>[8x]GNSITSATDEQPHIGNYRLQKTIGKG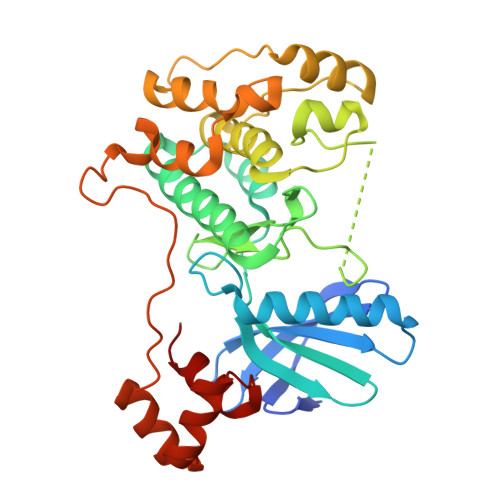NFAKVKLARHVLTGREVAVKIIDKTQLNPTSLQKLFREVRIMKILNHPNIVKLFEVIETEKTLYLVMEYASGGEVFDYLVAHGRMKEKEARAKFRQIVSAVQYCHQKYIVHRDLKAENLLLDGDMNIKIADFGFSNEFTVGNKLDTFCGSPPYAAPELFQGKKYDGPEVDVWSLGVILYTLVSGSLPFDGQNLKELRERVLRGKYRIPFYMSTDCENLLKKLLVLNPIKRGSLEQIMKDRWMNVGHEEEELKPYTEPDPDFNDTKRIDIMVTMGFARDEINDALINQKYDEVMATYILLGRK>[4x]MRRVAVLGAGPSGLTAARYLKQAGFEVMVFERYHHVGGTWNYTDETWMSEDGRPVYSSMYQNL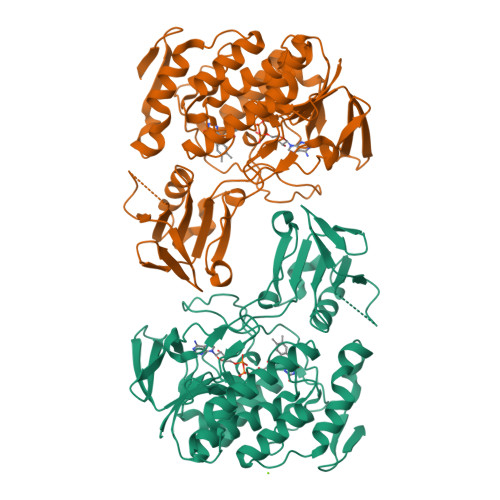FVNLPKELMAFPDFPFHDIEGSYVPSKEVLKYFDNFTDAFDLRKLIKLQHHVENVRPCESGWLVTVTDLTTMVEHSFEFDAVVVCTGQTWCPLYPDVEGRSFFRGRLTHAHEFRSPEPFRNKRVLIVGAGPSGHDMALHISYVSKEVFLSRKELKPVEGLFPDNVTEKPLLTSLSEYTAHFSDGTSTDVDEILYCTGYRYRFPFLSPECGVTVDEKYVYPLYLHMLNINKPTMLFIGVSYNACYSIMFDLQAQWVTAVLAGRCTLPDAETMRKEEAEYMEKQRAEAVHPHVLMNHQWEYFKKLEEMSGAKTMPPVYMKMFDDVASDLVKDLQNFRKNNYMIIDNENYKKIYAAALEHHHHHH Bacterial periplasmic binding proteins (PBP) are receptors for extracellular solutes in metabolite uptake, chemotaxis, and intercellular communication processes. The PBPs collectively constitute a structural protein superfamily characterized by two pseudo-symmetric domains that are linked by a hinge formed by two or three β-strands connecting the domains; a ligand-binding site is situated at the interface between the two domains. Solute binding induces a conformational change to form a closed state in which the ligand is bound at the domain interface and buried by the surrounding protein. We have characterized the stability, determined the ligand-binding properties, and solved the X-ray crystal structures of the apo and ligand-bound forms of a thermophilic periplasmic ribose-binding protein from the hyperthermophile Thermotoga maritima (tmRBP), the mesophilic homolog, ecRBP, of which has been studied in detail.

The apo-protein was crystallized using a construct that consisted of residues 30–310 (numbering according to NCBI NP 228766), containing a M142A mutation to prevent expression of the in-frame ORF. The construct used to crystallize the apo-form of tmRBP was a C-terminally truncated form of the protein (13 amino acids). However, superimposition of the tmRBP ribose complex C-terminal domain onto the C-terminal region of the apo protein suggests that these this region does not form interdomain interactions in the absence of ligand. The apo-protein and ribose-complex diffract to 1.4 Å and 2.15 Å resolution and were refined to Rcryst/Rfree values of 18.0/20.3 and 19.3/22.3 respectively. The apo-form of tmRBP was solved by separately searching with the amino- and carboxy-terminal domains of the ribose-bound form of tmRBP. However, the relative inter-domain angles differ significantly (43° for ecRBP; 28° and 20° for the two molecules in the tmRBP unit). The two molecules found in the tmRBP asymmetric unit differ in the inter-domain closure angle by 10°, analogous to the conformational heterogeneity observed in ecRBP. Molecule B is related to molecule A by a 10° closing about the hinge. This movement is limited to one of the two strands (residues 101–106) which connect the two domains. The positions of four bound water molecules are conserved (separated by less than 1.5Å in the aligned structures) in the open forms of ecRBP and tmRBP.

>[2x]MKGKMAIVISTLNNPWFVVLAETAKQRAEQLGYEATIFDSQNDTAKESAHFDAIIAAGYDAIIFNPTDADGSIANVKRAKEAGIPVFCVDRGINARGLAVAQIYSDNYYGGVLAGEYFVKFLKEKYPDAKEIPYAELLGILSAQPTWDRSNGFHSVVDQYPEFKMVAQQSAEFDRDTAYKVTEQILQAHPEIKAIWCGNDAMALGAMKACEAAGRTDIYIFGFDGAEDVINAIKEGKQIVATIMQFPKLMARLAVEWADQYLRGERSFPEIVPVTVELVTREGSHHHHHH> SNAMNDWASLGIGSIGEAVFSKLLKVVIDEAKKFKAFKPLSKDLVSTMEILFPLTQKIDSMQKELDFGVKELKELRDTIERADVAVRKFPRVKWYE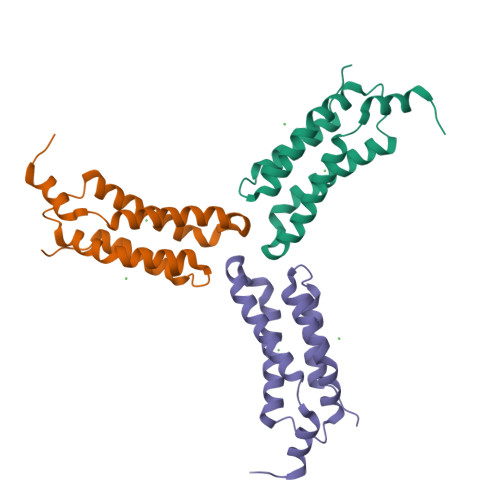ESEYTRKIERINKDMLKFCQIDLQLLQHRNQWSHPQFEK>[3x]MEDSPTMVRVDSPTMVRGENQVSPCQGRRCFPKALGYVTGDMKELANQLKDKPVVLQFIDWILRGISQVVFVNNPVSGILILVGLLVQNPWWALTGWLGTVVSTLMALLLSQDRSLIASGLYGYNATLVGVLMAVFSDKGDYFWWLLLPVCAMSMTCPIFSSALNSVLSKWDLPVFTLPFNMALSMYLSATGHYNPFFPAKLVIPITTAPNISWSDLSALELLKSIPVGVGQIYGCDNPWTGGIFLGD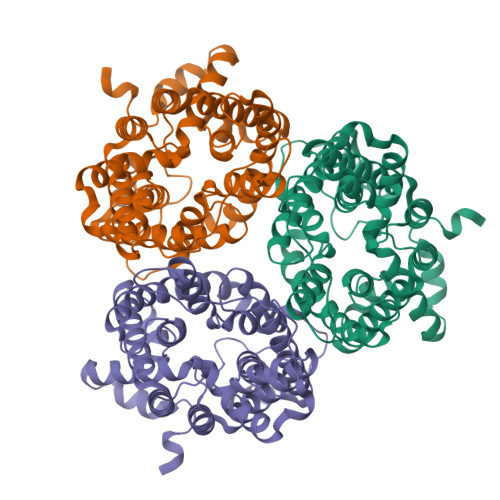ILLSSPLMCLHAAIGSLLGIAAGLSLSAPFENIYFGLWGFNSSLACIAMGGMFMALTWQTHLLALGCALFTAYLGVGMANFMAEVGLPACTWPFCLATLLFLIMTTKNSNIYKMPLSKVTYPEENRIFYLQAKKRMVESPL4-(4-fluorophenyl)piperazine-1-carboxamide 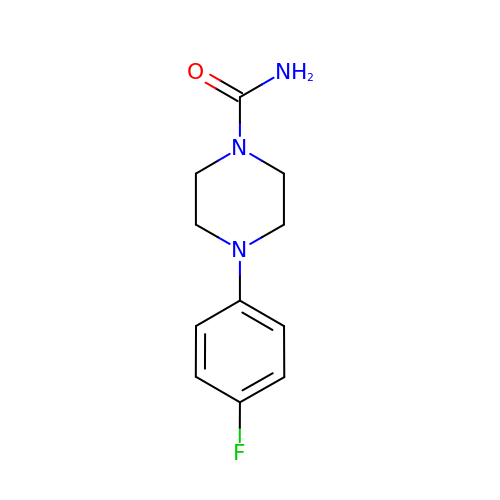| C11 H14 F N3 O | XARVCWHXIZRCGB-UHFFFAOYSA-N>GPGSMAATPLPPLRLAIACDDAGVSYKEALKAHLSDNPLVSSITDVGVTSTTDKTAYPHVAIQAAQLI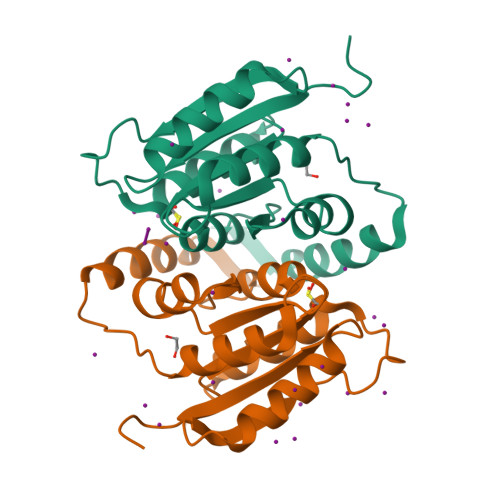KDGKVDRALMICGTGLGVAISANKVPGIRAVTAHDTFSVERAILSNDAQVLCFGQRVIGIELAKRLAGEWLTYRFDQKSASAQKVQAISDYEKKFVEVN[2x]(1S,2S,3S,4R,5R)-2-(benzylamino)-4-(phenylsulfanyl)-6,8-dioxabicyclo[3.2.1]octan-3-ol 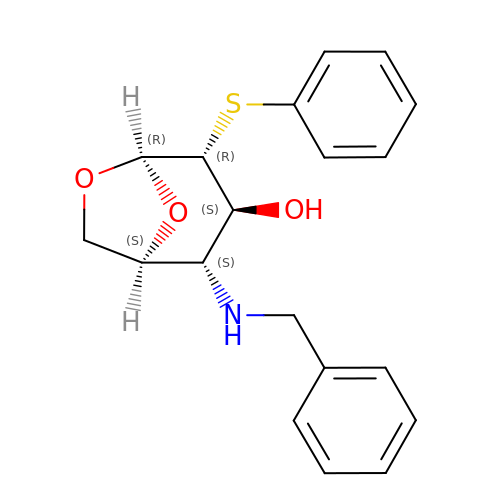| C19 H21 N O3 S | PZKNEARJFSZCKB-UJWQCDCRSA-N> SMEFQAALSRKVAELVHFLLLKYRAREPVTKAEMLGSVVGNWQYFFPVIFSKASSSLQLVFGIELMEVDPIGHLYIFATCLGLSYDGLLGDNQIMPKAGLLIIVLAIIAREGDCAPEEKIWEELSVLEVFEGREDSILGDPKKLLTQHFVQENYLEYRQVPGSDPACYEFLWGPRALVETSYVKVLHHMVKISGGPHISYPPLHEWVLREGEE

All MAGE family members contain a shared core MAGE homology domain (MHD) which is a ~ 200 amino acid long domain, which is well conserved across the entire MAGE family (individual human MHD’s share more than 40% sequence identity). The MHD domain structure consists of two highly modified winged helix WH domains WH1 and WH2 in a tandem arrangement linked by an extended β-hairpin. The biochemical basis for this activity appears to be exerted through binding to and modulating the activities of RING domain containing E3 ubiquitin ligases. Rather, each MAGE protein appears to recognize a unique region on its RING partner, suggesting that MAGE proteins are able to function as a versatile and adaptable protein interaction module.

Crystals of the MAGE-A3 MHD domain were obtained using a construct spanning residues 104–314, and diffracted to 2.0 Å resolution at Diamond light source beamline I24. The structure was solved by molecular replacement using the experimentally phased structure of MAGE-A4 as a search model. The electron density map is of overall excellent quality with the entirety of the single molecule in the asymmetric unit being modelled with the exception of the final 4 residues at the C-terminus, which were not included in the final model due to disorder. The final 15 residues at the C-terminus form an extended peptide, with a short section of 310 helix, which in the MAGE-A3 crystals forms an extensive interaction with a neighbouring molecule related by 2-fold crystallographic symmetry. In MAGE-A3 the interface area is ~1650 Å2 per monomer, consists of a mixture of polar and non-polar residues, and includes 5 unique hydrogen bonds, 1 salt bridge and two prominent aromatic residues, Tyr 301 and Trp 307, that protrude deep in the groove and make extensive van der Waals interactions with hydrophobic residues. In contrast to MAGEA4, PISA analysis of MAGE-A3 identified two potential biologically relevant dimer interfaces. In addition to the peptide interface detailed above (“dimer A”) a second interface is formed almost entirely by interactions from the second WH domain. This interface (“dimer B”) is only slightly less extensive (~1400 Å2 of interface area versus ~1650 Å2) and is formed by the extended β-hairpin connecting the two WH domains, together with the third helix on the second WH domain (α6) and the extended loop regions immediately preceding and following it. Comparing this data to the calculated data obtained using the monomeric MAGE-A3, dimer A and dimer B models reveals a significantly better fit for dimer B than either dimer A or monomer, when comparing either in reciprocal or real space (chi2 of 1.99 versus 4.94 or 2.6 respectively). Taken together it is clear that MAGE-A3 is predominantly a dimer in solution and that dimer corresponds to dimer B, although it is possible that at higher concentrations these dimeric units may further associate via the C-terminal peptide to form larger open ended oligomers.>[4x]ASVHGTTYELLRRQGIDTVFGNPGSNELPFLKDFPED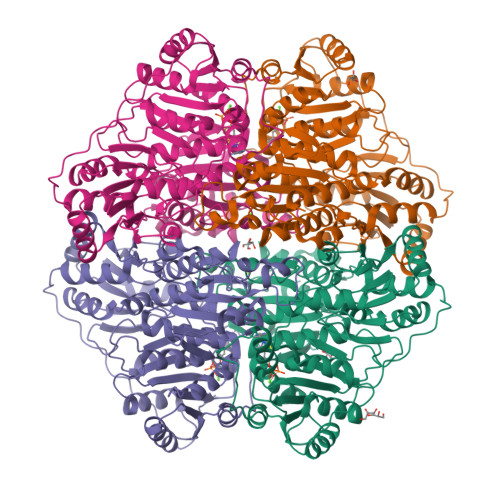FRYILALQEACVVGIADGYAQASRKPAFINLHSAAGTGNAMGALSNAWNSHSPLIVTAGQQTRAMIGVEALLTNVDAANLPRPLVKWSYEPASAAEVPHAMSRAIHMASMAPQGPVYLSVPYDDWDKDADPQSHHLFDRHVSSSVRLNDQDLDILVKALNSASNPAIVLGPDVDAANANADCVMLAERLKAPVWVAPSAPRCPFPTRHPCFRGLMPAGIAAISQLLEGHDVVLVIGAPVFRYYQYDPGQYLKPGTRLISVTCDPLEAARAPMGDAIVADIGAMASALANLVEESSRQLPTAAPEPAKVDQDAGRLHPETVFDTLNDMAPENAIYLNESTSTTAQMWQRLNMRNPGSYYFCAAGGLGFALPAAIGVQLAEPERQVIAVIGDGSANYSISALWTAAQYNIPTIFVIMNNGTYGILRWFAGVLEAENVPGLDVPGIDFRALAKGYGVQALKADNLEQLKGSLQEALSAKGPVLIEVSTVSPVKHHHHHH> NPSNSDAAHAFWSTQPVPQTEDETEKIVFAGPMDEPKTVADIPEEPYPIASTFEWWTPNMEAADDIHAIYELLRDNYVEDDDSMFRFNYSEEFLQWALCPPNYIPDWHVAVRRKADKKLLAFIAGVPVTLRMGTPKYMKVKAQEKGEGEEAAKYDEPRHICEINFLCVHKQLREKRLAPILIKEATRRVNRTNVWQAVYTAGVLLPTPYASGQYFHRSLNPEKLVEIRFSGIPAQYQKFQNPMAMLKRNYQLPSAPKNSGLREMKPSDVPQVRRILMNYLDSFDVGPVFSDAEISHYLLPRDGVVFTYVVENDKKVTDFFSFYRIPSTVIGNSNYNLLNAAYVHYYAATSIPLHQLILDLLIVAHSRGFDVCNMVEILD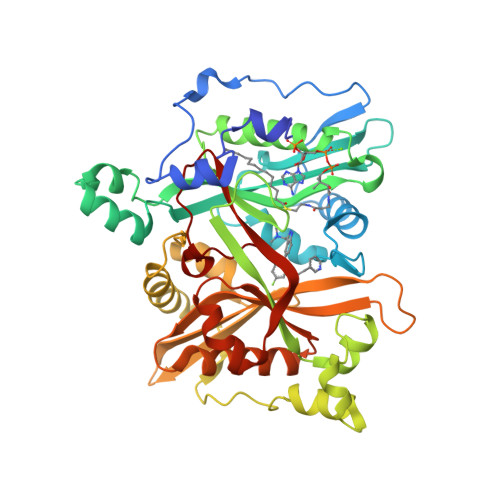NRSFVEQLKFGAGDGHLRYYFYNWAYPKIKPSQVALVML>SQLLNYIDGNFVTSASSFANINPVNGKLISDVFEADAKQVNEAVVAAQNALKGPWGKLSVQDRAALIHKIADGIQARFEEFVAAEVADTGRPVHQARTLDIPRAIANFRTFADLAKTSHTDLFEMSTSDGSGALNYTVRKPLGVIGVISPWNLPLLLFTWKVAPALACGNTVVAKPSEESPSSATLLAEVMHDAGVPPGVFNLIHGFGKDSAGEFLTQHPGISALTFTGESKTGSTIMKAVADGVKEVSFELGGKNAAVVFADADLDAAIEGVLRSSFTNSGQVCLCSERVYVHRSIFDEFVSGLKVEAERLVVGYPDQDGVNMGPLISHG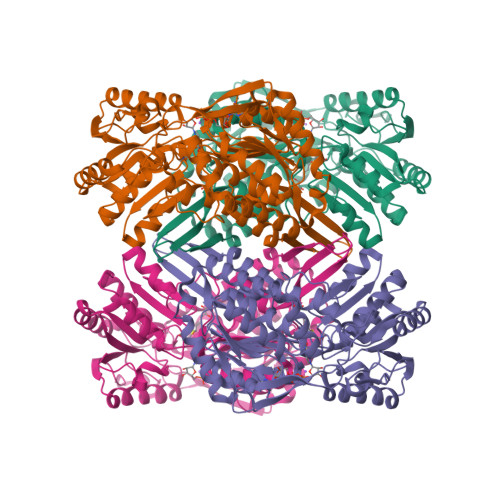HRDKVLSYYRLAVDEGATVVTGGGVPKFNDERDQGAYVQPTIWTGLSDKARCVTEEIFGPVCHISPFDDEDEVINRVNDSNYGLACAIWTTNLSRAHRVSRQIHVGLVWVNTWYLRDLRTPFGGVKLSGLGREGGRFSMDFYSDIANICIKI[4x]> MEFGFWSALYIFVLTCFLGYELITRVPVILHTPLMSGSNFIHGVVVVGAMVVLGHAETGLEKLIGFLGVILGAANAAGGYAVTVRMLEM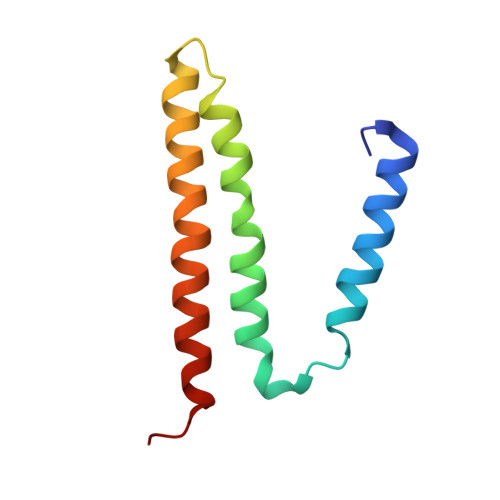FERKP>MQHTYPAQLMRFGTAARAEHMTIAAAIHALDADEADAIVMDIVPDGERDAWWDDEGFSSSPFTKNAHHAGIVATSVTLGQLQREQGDKLVSKAAEYFGIACRVNDGLRTTRFVRLFSDALDAKPLTIGHDYEVEFLLATRRVYEPFEAPFNFAPHCDDVSYGRDTVNWPLKRSFPRQLGGFLTIQGADNDAGMVMWDNRPESRAALDEMHAEYRETGAIAALERAAKIMLKPQPGQLTLFQSKNLHAIERCTSTRRTMGLFLIHTEDGWRMFD[2x]

SadA is a member of the dioxygenase family from Burkholderia ambifaria AMMD. This enzyme is useful as a novel biocatalyst for the (R)-selective hydroxylation at the C-3 position of N-substituted branched-chain L-amino acids, especially N-succinyl-L-leucine (NSLeu), to produce N-succinyl-(2S,3R)-3-hydroxyleucine (NSHLeu) with >99% stereoselectivity. One of the oxygen atoms is incorporated into the substrate to form hydroxy amino acid, while the other oxygen atom is used to oxidatively break down α-KG into succinate and CO2. This family of enzymes possesses a common protein fold, which is called the double-stranded β-helix (DSBH) fold, as the core of the structure, and an HXD/EXnH motif in the active site to coordinate the Fe(II) cofactor. The hydroxylation of amino acids is catalyzed by the ferrous [Fe(II)]- and α-ketoglutarate (α-KG)-dependent dioxygenases.

The crystal structures of SadA.Zn(II) and SadA.Zn(II).α-KG were determined at 1.77 Å and 1.98 Å resolutions, respectively. The structure of SadA.Zn(II) contained 11 β-strands, 6 α-helices and one 310 helix, and possessed the DSBH fold at its core, which was adopted in most of the α-KG-dependent dioxygenases. The DSBH fold of SadA was comprised of seven β-strands, four of which (β3, β5, β8 and β10) formed a major β-sheet and the other three of which (β6, β7 and β9) constituted a minor β-sheet. The β1, β2, β4 and β11 strands extended the major β-sheet. Six α-helices (α1-α6) were packed along the major β-sheet of the DSBH fold. The electron density maps of residues Ser60–Thr74 and Ala148–Phe152 were not observed in either of the structures. The data from inductively coupled plasma atomic emission spectroscopy (ICP-AES) showed that the concentration of Zn(II) was about 14-fold higher than that of Fe(II) in the SadA solution; therefore, the metal was modeled as Zn(II) substituting for Fe(II). Zn(II) is coordinated by the side chains of His155, Asp157 and His246, which are conserved in the dioxygenase superfamily. The dimers of SadA.Zn(II) and SadA.Zn(II).α-KG are structurally identical within 0.17 Å r.m.s.d. for 444 Cα atoms.>SMSPNGNLIRMLVLFFLESELHEHAAYLVDSLWESSQELLKDWECMTELLLEEPVQGEEAMSDRQESALIELMVCTIRQAAEAHPPVGRGTGKRVLTAKERKTQIDDRNKLTEHFIITLPMLLSKYSADAEKVANLLQIPQYFDLEIYSTGRMEKHLDALLKQIKFVVEKHVESDVLEACSKTYSILCSEEYTIQNRVDIARSQLIDEFVDRFNHSVEDLLQEGEEADDDDIYNVLSTLKRLTSFHNAHDLTKWDLFGNCYRLLKTGIEHGAMPEQIVVQALQCSHYSILWQLVKITDGSPSKEDLLVLRKTVKSFLAVCQQCLSNVNTPVKEQAFMLLCDLLMIFSHQLMTGGREGLQPLVFNP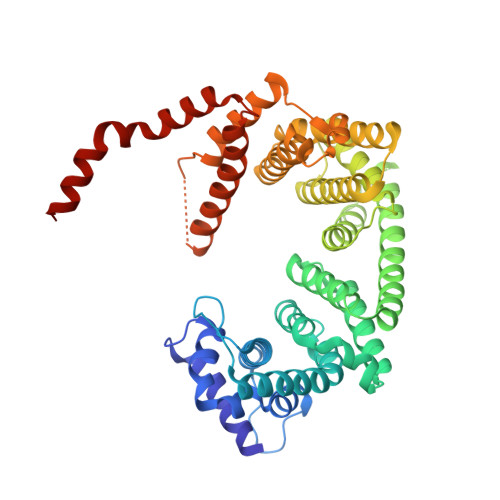DTGLQSELLSFVMDHVFIDQDEENQSMEGDEEDEANKIEALHKRRNLLAAFSKLIIYDIVDMHAAADIFKHYMKYYNDYGDIIKETLSKTRQID[2x]> MSNAKERKHAKKMRNQPTNVTLSSGFVADRGVKHHSGGEKPFQAQKQEPHPGTSRQRQTRVNPHSLPDPEVNEQSSSKGMFRKKGGWKAGPEGTSQEIPKYITASTFAQARAAEISAMLKAVTQKSSNSLVFQTLPRHMRRRAMSHNVKRLPRRLQEIAQKEAEKAVHQKKEHSKNKCHKARRCHMNRTLEFNRRQKKNIWLETHIWHAKRFHMVKKWGYCLGERPTVKSHRACYRAMTNRCLLQDLSYYCCLELKGKEEEILKALSGMCNIDTGLTFAAVHCLSGKRQGSLVLYRVNKYPREMLGPVTFIWKSQRTPGDPSESRQLWIWLHPTLKQDILEEIKAACQCVEPIKSAVCIADPLPTPSQEKSQTELPDEKIGKKRKRKDDGENAKPIKKIIGDGTRDPCLPYSWISPTTGIIISDLTMEMNRFRLIGPLSHSILTEAIKAASVHTVGEDTEETPHRWWIETCKKPDSVSLHCRQEAIFELLGGITSPAEIPAGTILGLTVGDPRINLPQKKSKALPNPEKCQDNEKVRQLLLEGVPVECTHSFIWNQDICKSVTENKISDQDLNRMRSELLVPGSQLILGPHESKIPILLIQQPGKVTGEDRLGWGSGWDVLLPKGWGMAFWIPFIYRGVRVGGLKESAVHSQYKRSPNVPGDFPDCPAGMLFAEEQAKNLLEKYKRRPPAKRPNYVKLGTLAPFCCPWEQLTQDWESRVQAYEEPSVASSPNGKESDLRRSEVPCAPMPKKTHQPSDEVGTSIEHPREAEEVMDAGCQESAGPERITDQEASENHVAATGSHLCVLRSRKLLKQLSAWCGPSSEDSRGGRRAPGRGQQGLTREACLSILGHFPRALVWVSLSLLSKGSPEPHTMICVPAKEDFLQLHEDWHYCGPQESKHSDPFRSKILKQKEKKKREKRQKPGRASSDGPAGEEPVAGQEALTLGLWSGPLPRVTLHCSRTLLGFVTQGDFSMAVGCGEALGFVSLTGLLDMLSSQPAAQRGLVLLRPPASLQYRFARIAIEV;> MAAAPQAPGRGSLRKTRPLVVKTSLNNPYIIRWSALESEDMHFILQTLEDRLKAIGLQKIEDKKKKNKTPFLKKESREKCSIAVDISENLKEKKTDAKQQVSGWTPAHVRKQLAIGVNEVTRALERRELLLVLVCKSVKPAMITSHLIQLSLSRSVPACQVPRLSERIAPVIGLKCVLALAFKKNTTDFVDEVRAIIPRVPSLSVPWLQDRIEDSGENLETEPLESQDRELLDTSFEDLSKPKRKLADGRQASVTLQPLKIKKLIPNPNKIRKPPKSKKATPK;> MKSVIYHALSQKEANDSDVQPSGAQRAEAFVRAFLKRSTPRMSPQAREDQLQRKAVVLEYFTRHKRKEKKKKAKGLSARQRRELRLFDIKPEQQRYSLFLPLHELWKQYIRDLCSGLKPDTQPQMIQAKLLKADLHGAIISVTKSKCPSYVGITGILLQETKHIFKIITKEDRLKVIPKLNCVFTVETDGFISYIYGSKFQLRSSERSAKKFKAKGTIDL;> MVRFKHRYLLCELVSDDPRCRLSLDDRVLSSLVRDTIARVHGTFGAAACSIGFAVRYLNAYTGIVLLRCRKEFYQLVWSALPFITYLENKGHRYPCFFNTLHVGGTIRTCQKFLIQYNRRQLLILLQNCTDEGEREAIQKSVTRSCLLEEEEESGEEAAEAME;> MENFRKVRSEEAPAGCGAEGGGPGSGPFADLAPGAVHMRVKEGSKIRNLMAFATASMAQPATRAIVFSGCGRATTKTVTCAEILKRRLAGLHQVTRLRYRSVREVWQSLPPGPTQGQTPGEPAASLSVLKNVPGLAILLSKDALDPRQPGYQPPNPHPGPSSPPAAPASKRSLGEPAAGEGSAKRSQPEPGVADEDQTA;> MAENREPRGAVEAELDPVEYTLRKRLPSRLPRRPNDIYVNMKTDFKAQLARCQKLLDGGARGQNACSEIYIHGLGLAINRAINIALQLQAGSFGSLQVAANTSTVELVDELEPETDTREPLTRIRNNSAIHIRVFRVTPK;> MPAPAATYERVVYKNPSEYHYMKVCLEFQDCGVGLNAAQFKQLLISAVKDLFGEVDAALPLDILTYEEKTLSAILRICSSGLVKLWSSLTLLGSYKGKKCAFRVIQVSPFLLALSGNSRELVLD;>MAVFADLDLRAGSDLKALRGLVETAAHLGYSVVAINHIVDFKEKKQEIEKPVAVSELFTTLPIVQGKSRPIKILTRLTIIVSDPSHCNVLRATSSRARLYDVVAVFPKTEKLFHIACTHLDVDLVCITVTEKLPFYFKRPPINVAIDRGLAFELVYSPAIKDSTMRRYTISSALNLMQICKGKNVIISSAAERPLEIRGPYDVANLGLLFGLSESDAKAAVSTNCRAALLHGETRKTAFGIISTVKKPRPSEGDEDCLPASKKAKCEG[2x];> MAGPVKDREAFQRLNFLYQAAHCVLAQDPENQALARFYCYTERTIAKRLVLRRDPSVKRTLCRGCSSLLVPGLTCTQRQRRCRGQRWTVQTCLTCQRSQRFLNDPGHLLWGDRPEAQLGSQADSKPLQPLPNTAHSISDRLPEEKMQTQGSSNQ;> MATLRRLREAPRHLLVCEKSNFGNHKSRHRHLVQTHYYNYRVSFLIPECGILSEELKNLVMNTGPYYFVKNLPLHELITPEFISTFIKKGSC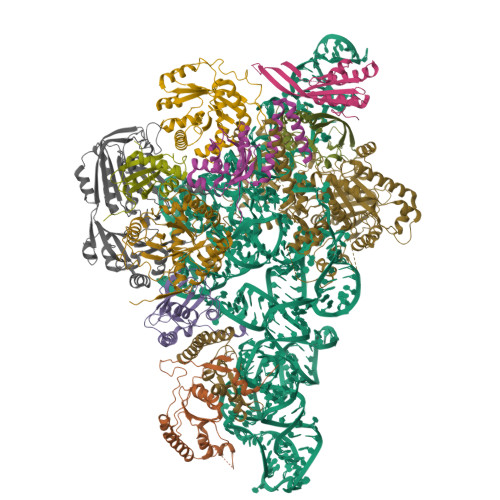YALTYNTHIDEDNTVALLPNGKLILSLDKDTYEETGLQGHPSQFSGRKIMKFIVSIDLMELSLNLDSKKYERISWSFKEKKPLKFDFLLAWHKTGSEESTMMSYFSKYQIQEHQPKVALSTLRDLQCPVLQSSELEGTPEVSCRALELFDWLGAVFSNVDLNNEPNNFISTYCCPEPSTVVAKAYLCTITGFILPEKICLLLEHLCHYFDEPKLAPWVTLSVQGFADSPVSWEKNEHGFRKGGEHLYNFVIFNNQDYWLQMAVGANDHCPP> ASSFVQTSGPQFTLDGKPFYFEGTNAYYLMTSDQSNVKQVFSDMKSLGLPVVRTWLFNLGSDSVWFQQWDSSSNKMVINDNSDTGLGRIDYIIQQAASQDIKLIFTLNNNWEDYGGMDYYVKNFGGTY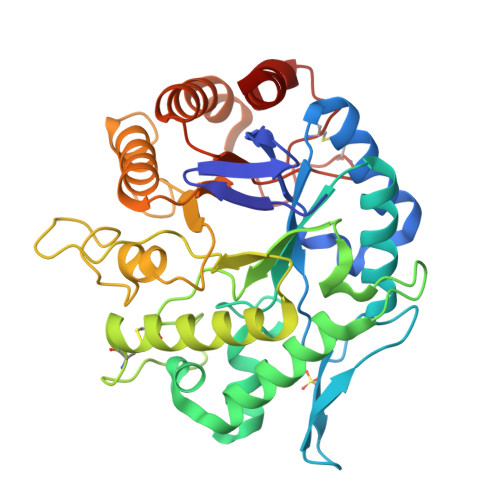HDDFYTNTEMIDSFKEYISHVLNRENSLTGVKYKDDPTIFGWEIANEPRCVGSGDFPASSNCSTTVTTAWIKEISEYIKSIDSNHLVAVGDEGFFNRKGESDYEYNGGSGMDFDAILALSSIDFGTFHLYPEAWSKGTDSSWSVQWIKDHAAAQADADKPVIMEEYGLSTDALRVAQYPVWQGTVEDEDLAADAFWQIAVPCSTMDGFGICASDNDIATTVTNHADAMAKK> SMFLPPPECPVFEPSWEEFADPFAFIHKIRPIAEQTGICKVRPPPDWQPPFACDVDKLHFTPRIQRLNELEAQTRVKLGGGGAKDYTLRTFGEMADAFKSDYFNMPVHMVPTELVEKEFWRLVSTIEEDVTVEYGADIASKEFGSGFPVRDGKIKLSPEEEEYLDSGWNLNNMPVMEQSVLAHITADICGMKLPWLYVGMCFSSFCWHIEDHWSYSINYLHWGEPKTWYGVPGYAAEQLENVMKKLAPELFVSQPDLLHQLVTIMNPNTLMTHEVPVYRTNQCAGEFVITFPRAYHSGFNQGFNFAEAVNFCTVDWLPLGRQCVEHYRLLHRYCVFSHDE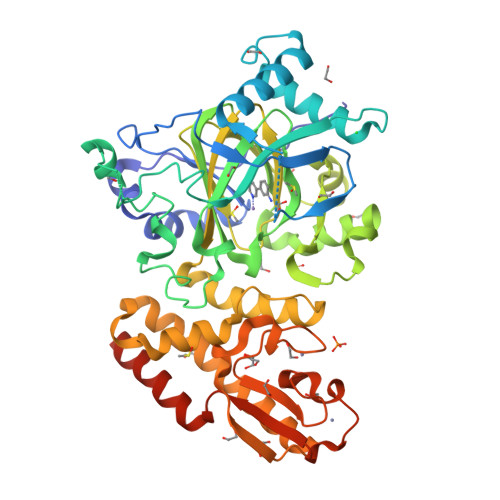MICKMASKADVLDVVVASTVQKDMAIMIEDEKALRETVRKLGVIDSERMDFELLPDDERQCVKCKTTCFMSAISCSCKPGLLVCLHHVKELCSCPPYKYKLRYRYTLDDLYPMMNALKLRAESYNEWALNVNEALEAKI>GSHMGGVEVLEVKTGVDSITEVECFLTPEMGDPDEHLRGFSKSISISDTFESDSPNKDMLPCYSVARIPLPNLNEDLTCGNILMWEAVTLKTEVIGVTTLMNVHSNGQATHDNGAAKPVQGTSFHFFSV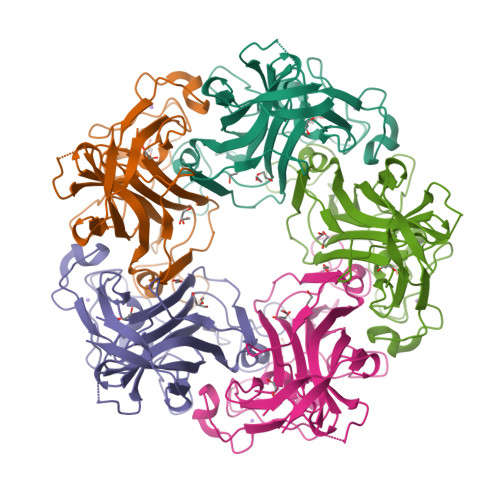GGEALELQGVVFNYRTTYPDGTIFPKNATVQSQVMNTEHKAYLDKNKAYPVECWVPDPTRNENTRYFGTLTGGENVPPVLHITNTATTVLLDEFGVGPLCKGDNLYLSAVDVCGMFTNRSGSQQWRGLSRYFKVQLRKRRVKN[5x]>SNAMNRIEHYHDWLRDAHAMEKQAESMLESMASRIDNYPELRARIEQH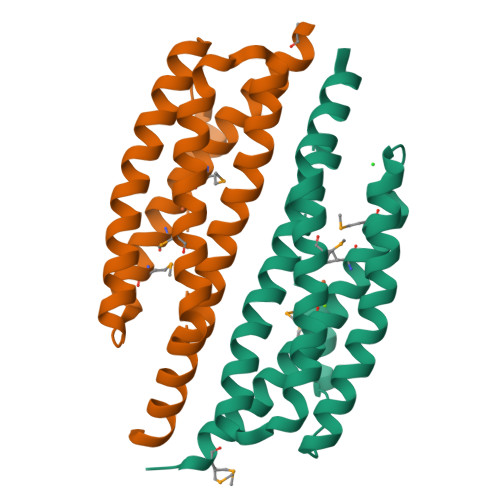LSETKNQIVQLETILDRNDISRSVIKDSMSKMAALGQSIGGIFPSDEIVKGSISGYVFEQFEIACYTSLLAAAKNAGDTASIPTIEAILNEEKHMADWLIQHIPQTTEKFLIRSETDGVEAKK[2x]> SASASAMLSRKGIIPEEYVLTRLAEDPAEPRYRARQRRARFVSKKGNCNVAHKNIREQGRFLQDVFTTLVDLKWPHTLLIFTMSFLCSWLLFAMAWWLIAFAHGDLAPSEGTAEPCVTSIHSFSSAFLFSIEVQVTIGFGGRMVTEECPLAILILIVQNIVGLMINAIMLGCIFMKTAQAHRRAETLIFSKHAVIALRHGRLCFMLRVGDLRKSMIISA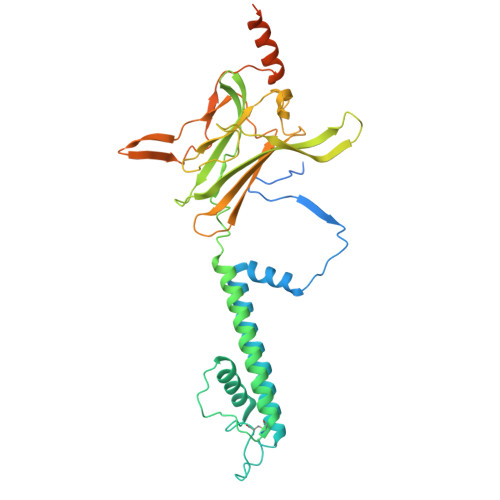TIHMQVVRKTTSPEGEVVPLHQVDIPMENGVGGNSIFLVAPLIIYHVIDANSPLYDLAPSDLHHHQDLEIIVILEGVVETTGITTQARTSYLADEILWGQRFVPIVAEEDGRYSVDYSKFGNTIKVPTPLCTARQLDEDHSLLEALTLASARGPLRKRSVPMAKAKPKFSISPDSLSSNSLEVLFQG>[60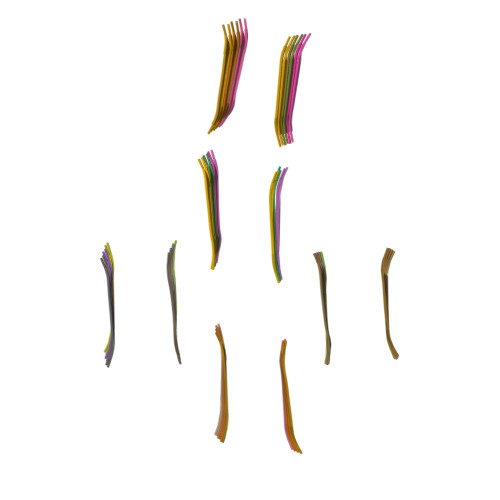x]TLKIVWI> GEFELMSIKEELMEIIEAIKYTSEKPEEIVHGKGPRIIVKESRIIDVQGDEGIILEGKEEDGKIKAKIIVKKGYKFKYPIHMCFGITEENISQIIDVEIILEEDSSISLMSHCSFP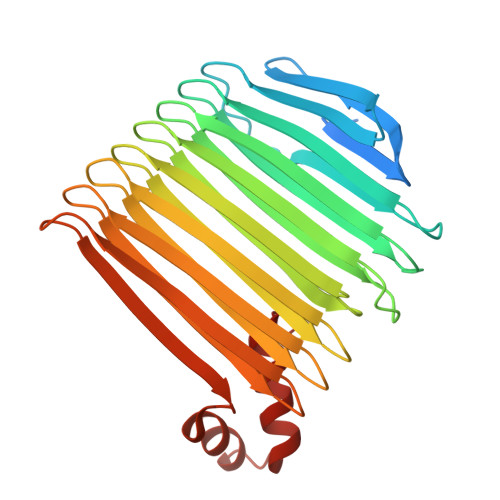KGKGIKHIMNGIIKIGKNAKFSYNEFHYHGMDGDILVKPTVKVEIDEGGIYISNFTLTKGRIGTLDIEQEIIAKKDAIIDITTRTYAIKEDVVKVNEVVKLNGENAKCIIKSRGAAMDNSKISLKLKIEGNAPYSKGHIDCAEIVKGNAEVESIPIVVVRDDKARITHEAAIGSVDKKQLETLMAKGLDEDEATEIIVKGMIGDL> GSKPHQWQADEEAVRSATCSFSVKYLGCVEVFESRGMQVCEEALKVLRQSRRRPVRGLLHVSGDGLRVVDDETKGLIVDQTIEKVSFCAPDRNHERGFSYICRDGTTRRWMCHGFLACKDSGERLSHAVGCAFAVCLERKQ;> KKKKREHACFENPGL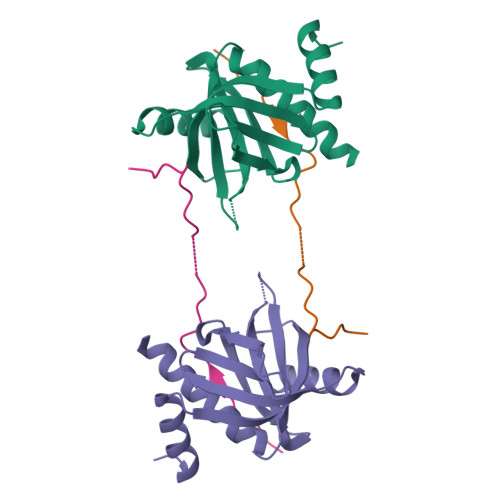NLELPEKQFNPYEVVRSA>[2x]TDKLTSLRQYTTVVADTGDIAAMKLYQPQDATTNPSLILNAAQIPEYRKLIDDAVAWAKQQSNDRAQQIVDATDKLAVNIGLEILKLVPGRISTEVDARLSYDTEASIAKAKRLIKLYNDAGISNDRILIKLASTWQGIRAAEQLEKEGINCNLTLLFSFAQARACAEAGVFLISPFVGRI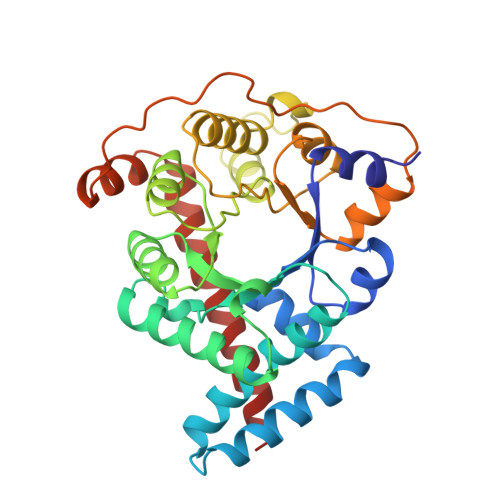LDWYKANTDKKEYAPAEDPGVVSVSEIYQYYKEHGYETVVMGASFRNIGEILELAGCDRLTIAPALLKELAESEGAIERKLSYTGEVKARPARITESEFLWQHNQDPMAVDKLAEGIRKFAIDQEKLEKMIGDLL>[2x]MEHYDLAIIGTGSGNSIVDDRYAGKKVAICEQGTFGGTCLNVGCIPTKMFVYAAEVAHSVRTSARYGVDAHIDKVRWPDIVERVFGRIDPIAAGGEDYRRSDPNITVYSSHTRFGPKTDDGRYTLRTESGEEFTSDQVVIAAGSRTYIPPAVVDCGVKYHTSDDIMRIPELPTDLVIIGGGFVSAEFAHVFSALGVHVTIVVRGDGLLTHCDETICHRFNEIAATKWDIRTHENVIGSH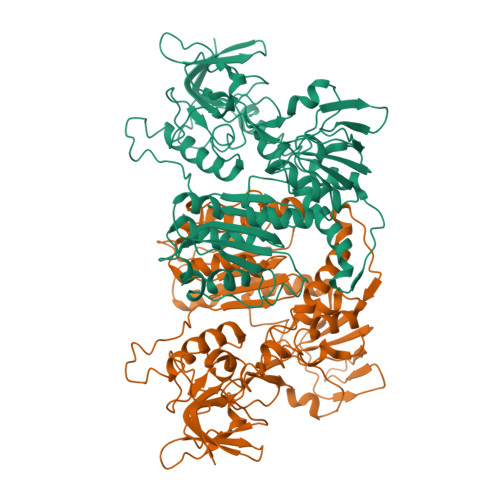QDGDRIVLELDDGKTVAADTLLVATGRVPNGDLLDAELAGVEVDEDGRVIVDQYQRTTARGVFALGDVSSDYQLKHVANHEARVVKENLLRDWDDTASLVASDHRFVPSAVFTDPQVATVGLTEAEARAAGHDIVVKVQNYGDTAYGWAMEDTTGIAKLIGERGTGKLLGAHILGHQASSIIQPLIQAMSLGQTAQEIARGQYWIHPALPEVIENALLGLQE>GMSVPTLPTGPTVDLAQAAERLIKGRRAVRAFRPDEVPEETMRAVFELAGHAPSNSNTQPWHVEVVSGAARDRLAEALVTAHAEERVTVDFPYREGLFQGVLQERRADFGSRLYAALGIARDQTDLLQGYNTESLRFYGAPHVAMLFAPNNTEARIAGDMGIYAQTLMLAMTAHGIASCPQALLSFYADTVRAELGVENRKLLMGIS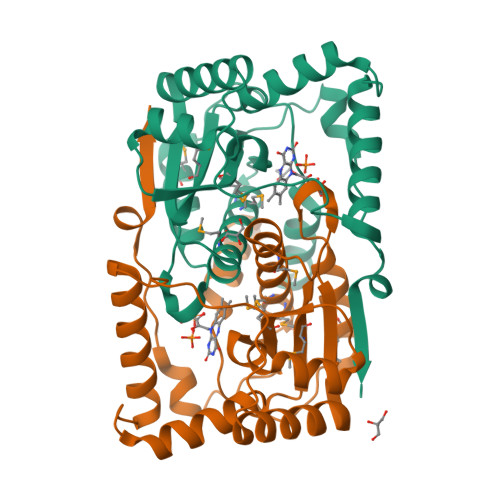FGYADDTAAVNGVRIPRAGLSETTRFSR[2x]> MGSSHHHHHHSSGRENLYFQGHMLFISATNTNAGKTTCARLLAQYCNACGVKTILLKPIETGVNDAINHSSDAHLFLQDNRLLDRSLTLK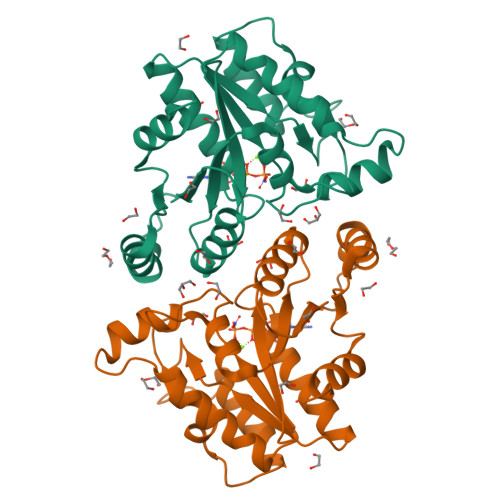DISFYRYHKVSAPLIAQQEEDPNAPIDTDNLTQRLHNFTKTYDLVIVEGAGGLCVPITLEENMLDFALKLKAKMLLISHDNLGLINDCLLNDFLLKSHQLDYKIAINLKGNNTAFHSISLPYIELFNTRSNNPIVIFQQSLKVLMSFALKGS> GPGELAYALNNFDKQIIVDPLSF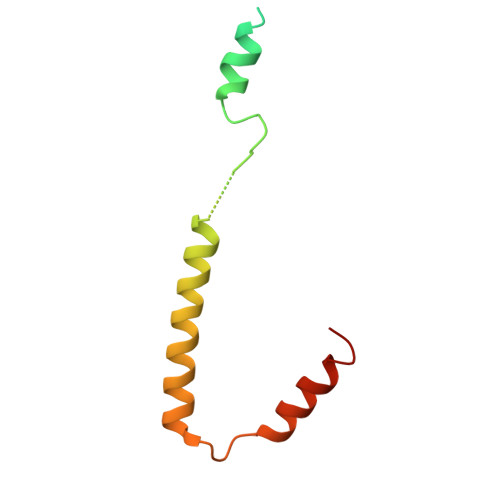SEERFRPSLEERLESIISGAALMADSSCTRDDRRERIVAECNAVRQALQDLLSEYMGNAGRKERSDALNSAIDKMTKKT> GPLGSM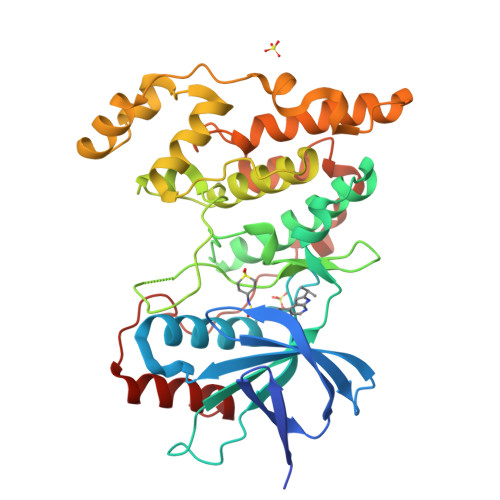SRSKRDNNFYSVEIGDSTFTVLKRYQNLKPIGSGAQGIVCAAYDAILERNVAIKKLSRPFQNQTHAKRAYRELVLMKCVNHKNIIGLLNVFTPQKSLEEFQDVYIVMELMDANLCQVIQMELDHERMSYLLYQMLCGIKHLHSAGIIHRDLKPSNIVVKSDCTLKILDFGLARTAGTSFMMTPYVVTRYYRAPEVILGMGYKENVDLWSVGCIMGEMVCHKILFPGRDYIDQWNKVIEQLGTPCPEFMKKLQPTVRTYVENRPKYAGYSFEKLFPDVLFPADSEHNKLKASQARDLLSKMLVIDASKRISVDEALQHPYINVWYDPSEAEAPPPKIPDKQLDEREHTIEEWKELIYKEVMDLE> MVILGVGYFLLGLILLYYGSDWFVLGSERIARHFNVSNFVIGATVMAIGTSLPEILTSAYASYMHAPGISIGNAIGSCICNIGLVLGLSAIISPIIVDKNLQKNILVYLLFVIFAAVIGIDGFSWIDGVVLLILFIIYLRWTVKNGSAEIEENNDKNNPSVVFSLVLLIIGLIGVLVGAELFVDGAKKIALALDISDKVIGFTLVAFGTSLPELMVSLAAAKR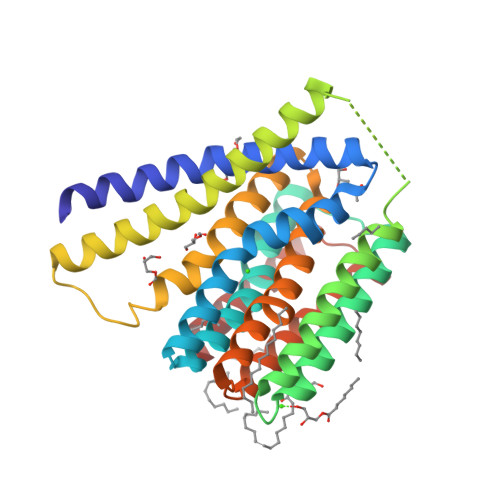NLGGMVLGNVIGSNIADIGGALAVGSLFMHLPAENVQMAVLVIMSLLLYLFAKYSKIGRWQGILFLALYIIAIASLRMG> MTDVA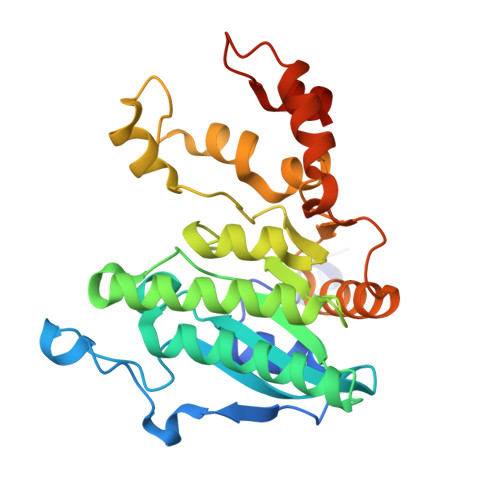RLLALRSFTELGARQRARALLDAGSFRELLDPFAGVQSPWLERQGIVPQADDGVVVARGLLDGQPAVLAAIEGAFQGGSLGEVSGAKIAGALELAAEDNRNGVPTRALLLLETGGVRLQEANLGLAAIAEIQAAIVDLQRYQPVVAVIAGPVGCFGGMSIAAGLCSYVLVTREARLGLNGPQVIEQEAGIAEYDSRDRPFIWSLTGGEQRFASGLADAYLADDLDEVRTSVLAYFAKGLPARPRCRRAEDYLRRLGDLDTAEQPDAAGVRRLYQGLGQGDAT VZV belongs to the Alphaherpesvirinae subfamily of Herpesviridae, a group of enveloped double-stranded DNA (dsDNA) viruses. The highly organized dsDNA genome is enclosed in an icosahedral capsid shell comprised by multiple viral proteins, which protects the viral genome from being exposed to the extracellular environment or detected by immune sensors in the cytosol. In the replication process, the viral capsid plays a central role in maintaining viral genome integrity and enabling virion assembly in a highly regulated manner. Similar to other herpesvirus capsids, the VZV capsid is composed mainly of four types of protein that are arranged in icosahedral symmetry with a triangulation (T) number of 16, including the major capsid protein (MCP), the small capsid protein (SCP), and the Tri1 and Tri2 proteins that make up the heterotriplex.

In this work, we present the 3.7-Å-resolution structure of the VZV A-capsid determined by cryogenic electron microscopy (cryo-EM) single-particle reconstruction. To counteract the effects of local defocus variation and conformational heterogeneity within the large capsid particle, localized reconstruction of the sub-particles was carried out to resolve better details within an asymmetric unit (ASU). This strategy improved the resolution of the ASU block to 3.7 Å, in which most regions of the capsid floor reached a local resolution of 3.5 Å and the apical regions of the capsomer spikes revealed a relatively lower resolution of 4.0–4.5 Å. Each ASU contains 16 MCPs, 15 SCPs, and 5 heterotriplexes (Ta–Te). The MCPs assemble into either pentamers (pentons) at the 5-fold vertex or hexamers (hexons) in each facet of the icosahedron. On top of each hexon, six SCPs form a cap to cover the upper crown and to bridge adjacent MCP protomers for securing the hexameric structure. By contrast, SCPs are not present in the penton capsomer of the VZV capsid. Additionally, the N-lasso is well resolved in hexon MCPs, whereas it is disordered in the pentons, resulting in loss of the lasso interactions between the pentons and adjacent P-hexons. The heterotriplex consists of one Tri1 and two Tri2 subunits that are assembled into a triangular-shaped structure. The embracing arms adopt different conformations in the two protomers, which are further crosslinked by an interchain disulfide bond.

>[16x]MTTVSCPANVITTTESDRIAGLFNIPAGIIPTGNVLSTIEVCAHRCIFDFFKQIRSDDNSLYSAQFDILLGTYCNTLNFVRFLELGLSVACICTKFPELAYVRDGVIQFEVQQPMIARDGPHPVDQPVHNYMVKRIHKRSLSAAFAIASEALSLLSNTYVDGTEIDSSLRIRAIQQMARNLRTVLDSFERGTADQLLGVLLEKAPPLSLLSPINKFQPEGHLNRVARAALLSDLKRRVCADMFFMTRHAREPRLISAYLSDMVSCTQPSVMVSRITHTNTRGRQVDGVLVTTATLKRQLLQGILQIDDTAADVPVTYGEMVLQGTNLVTALVMGKAVRGMDDVARHLLDITDPNTLNIPSIPPQSNSDSTTAGLPVNARVPADLVIVGDKLVFLEALERRVYQATRVAYPLIGNIDITFIMPMGVFQANSMDRYTRHAGDFSTVSEQDPRQFPPQGIFFYNKDGILTQLTLRDAMGTICHSSLLDVEATLVALRQQHLDRQCYFGVYVAEGTEDTLDVQMGRFMETWADMMPHHPHWVNEHLTILQFIAPSNPRLRFELNPAFDFFVAPGDVDLPGPQRPPEAMPTVNATLRIINGNIPVPLCPISFRDCRGTQLGLGRHTMTPATIKAVKDTFEDRAYPTIFYMLEAVIHGNERNFCALLRLLTQCIRGYWEQSHRVAFVNNFHMLMYITTYLGNGELPEVCINIYRDLLQHVRALRQTITDFTIQGEGHNGETSEALNNILTDDTFIAPILWDCDALIYRDEAARDRLPAIRVSGRNGYQALHFVDMAGHNFQRRDNVLIHGRPVRGDTGQGIPITPHHDREWGILSKIYYYIVIPAFSRGSCCTMGVRYDRLYPALQAVIVPEIPADEEAPTTPEDPRHPLHAHQLVPNSLNVYFHNAHLTVDGDALLTLQELMGDMAERTTAILVSSAPDAGAATATTRNMRIYDGALYHGLIMMAYQAYDETIATGTFFYPVPVNPLFACPEHLASLRGMTNARRVLAKMVPPIPPFLGANHHATIRQPVAYHVTHSKSDFNTLTYSLLGGYFKFTPISLTHQLRTGFHPGIAFTVVRQDRFATEQLLYAERASESYFVGQIQVHHHDAIGGVNFTLTQPRAHVDLGVGYTAVCATAALRCPLTDMGNTAQNLFFSRGGVPMLHDNVTESLRRITASGGRLNPTEPLPIFGGLRPATSAGIARGQASVCEFVAMPVSTDLQYFRTACNPRGRASGMLYMGDRDADIEAIMFDHTQSDVAYTDRATLNPWASQKHSYGDRLYNGTYNLTGASPIYSPCFKFFTPAEVNTNCNTLDRLLMEAKAVASQSSTDTEYQFKRPPGSTEMTQDPCGLFQEAYPPLCSSDAAMLRTAHAGETGADEVHLAQYLIRDASPLRGCLPLPR;>MTQPASSRVVFDPSNPTTFSVEAIAAYTPVALIRLLNASGPLQPGHRVDIADARSIYTVGAAASAARARANHNANTIRRTAMFAETDPMTWLRPTVGLKRTFNPRIIRPQPPNPSMSLGISGPTILPQKTQSADQSALQQPAALAFSGSSPQHPPPQTTSASVGQQQHVVSGSSGQQPQQGAQSSTVQPTTGSPPAAQGVPQSTPPPTQNTPQGGKGQTLSHTGQSGNASRSRRV[15x];>[10x]MAMPFEIEVLLPGELSPAETSALQKCEGKIITFSTLRHRASLVDIALSSYYINGAPPDTLSLLEAYRMRFAAVITRVIPGKLLAHAIGVGTPTPGLFIQNTSPVDLCNGDYICLLPPVFGSADSIRLDSVGLEIVFPLTIPQTLMREIIAKVVARAVERTAAGAQILPHEVLRGADVICYNGRRYELETNLQHRDGSDAAIRTLVLNLMFSINEGCLLLLALIPTLLVQGAHDGYVNLLIQTANCVRETGQLINIPPMPRIQDGHRRFPIYETISSWISTSSRLGDTLGTRAILRVCVFDGPSTVHPGDRTAVIQV;>[5x]MGSQPTNSHFTLNEQTLCGTNISLLGNNRFIQIGNGLHMTYAPGFFGNWSRDLTIGPRFGGLNKQPIHVPPKRTETASIQVTPRSIVINRMNNIQINPTSIGNPQVTIRLPLNNFKSTTQLIQQVSLTDFFRPDIEHAGSIVLILRHPSDMIGEANTLTQAGRDPDVLLEGLRNLFNACTAPWTVGEGGGLRAYVTSLSFIAACRAEEYTDKQAADANRTAIVSAYGCSRMETRLIRFSECLRAMVQCHVFPHRFISFFGSLLEYTIQDNLCNITAVAKGPQEAARTDKTSTRRVTANIPACVFWDVDKDLHLSADGLKHVFLVFVYTQRRQREGVRLHLALSQLNEQCFGRGIGFLLGRIRAENAAWGTEGVANTHQPYNTRALPLVQLSNDPTSPRCSIGEITGVNWNLARQRLYQWTGDFRGLPTQLSCMYAAYTLIGTIPSESVRYTRRMERFGGYNVPTIWLEGVVWGGTNTWNECYY>MSRNTEATDDVKTWTGGPLNYKEGFFTQLATDELAKGINEEVVRAISAKRNEPEWMLEFRLNAYRAWLEMEEPHWLKAHYDKLNYQDYSYYSAPSCGNCDDTCASEPGAVQQT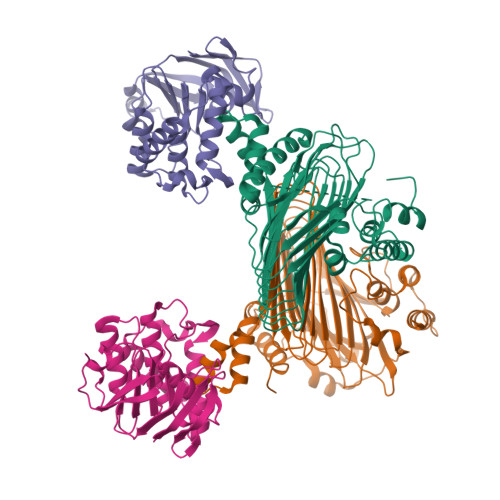GANAFLSKEVEAAFEQLGVPVREGKEVAVDAIFDSVSVATTYREKLAEQGIIFCSFGEAIHDHPELVRKYLGTVVPGNDNFFAALNAAVASDGTFIYVPKGVRCPMELSTYFRINAEKTGQFERTILVADEDSYVSYIEGCSAPVRDSYQLHAAVVEVIIHKNAEVKYSTVQNWFPGDNNTGGILNFVTKRALCEGENSKMSWTQSETGSAITWKYPSCILRGDNSIGEFYSVALTSGHQQADTGTKMIHIGKNTKSTIISKGISAGHSQNSYRGLVKIMPTATNARNFTQCDSMLIGANCGAHTFPYVECRNNSAQLEHEATTSRIGEDQLFYCLQRGISEEDAISMIVNGFCKDVFSELPLEFAVEAQKLLAISLEHSVG[2x];>MAGLPNSSNALQQWHHLFEAEGTKRSPQAQQHLQQLLRTGLPTRKHENWKYTPLEGLINSQFVSIAGEISPQQRDALALTLDSVRLVFVDGRYVPALSDATEGSGYEVSINDDRQGLPDAIQAEVFLHLTESLAQSVTHIAVKRGQRPAKPLLLMHITQGVAGEEVNTAHYRHHLDLAEGAEATVIEHFVSLNDARHFTGARFTINVAANAHLQHIKLAFENPLSHHFAHNDLLLAEDATAFSHSFLLGGAVLRHNTSTQLNGENSTLRINSLAMPVKNEVCDTRTWLEHNKGFCNSRQLHKTIVSDKGRAVFNGLINVAQHAIKTDGQMTNNNLLMGKLAEVDTKPQLEIYADDVKCSHGATVGRIDDEQIFYLRSRGINQQDAQQMIIYAFAAELTEALRDEGLKQQVLARIGQRLPGGAR[2x];>MLSIKDLHVSVEDKAILRGLSLDVHPGEVHAIMGPNGSGKSTLSATLAGREDYEVTGGTVEFKGKDLLALSPEDRAGEGIFMAFQYPVEIPGVSNQFFLQTALNAVRSYRGQETLDRFDFQDLMEEKIALLKMPEDLLTRSVNVGFSGGEKKRNDILQMAVLEPELCILDESDSGLDIDALKVVADGVNSLRDGKRSFIIVTHYQRILDYIKPDYVHVLYQGRIVKSGDFTLVKQLEEQGYGWLTEQQ[4x]>MGSDKIHHHHHHMIVEKVLIVDPIDGEFTGDVEIEEGKIVKVEKRECIPRGVLMPGFVDPHIHGVVGADTMNCDFSEMEEFLYSQGVTTFLATTVSTSLEKMKEILRKARDYILENPSTSLLGVHLEGPYISKEKKGAHSEKHIRPPSERELSEIDSPAKMLTFAPEIESSELLLRLVKRDIVLSAGHSIATFEEFMKFYKEGVKRITHFPNGLKPLHHREIGITGAGLLLDDVKLELICDGVHLSREMVKLVYKVKKANGIVLVTDSISAAGLKDGTTTLGDLVVKVKDGVPRLEDGTLAGSTLFFSQAVKNFRKFTGCSITELAKVSSYNSCVELGLDDRGRIAE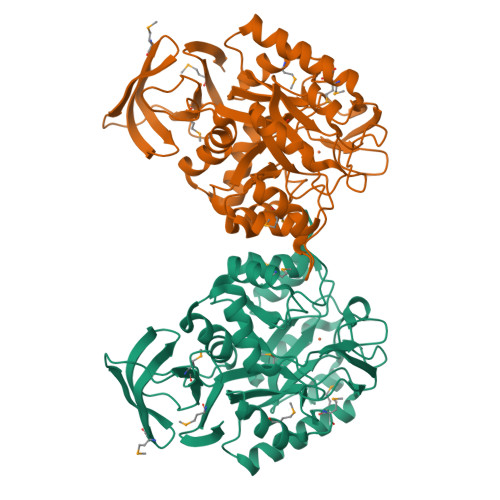GTRADLVLLDEDLNVVMTIKEGEVVFRSR[2x]[4-(2-chloro-4-nitrophenyl)piperazin-1-yl][3-(2-methoxyphenyl)-5-methyl-1,2-oxazol-4-yl]methanone 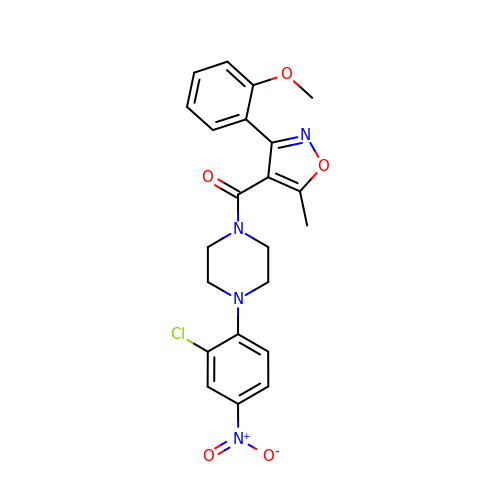| C22 H21 Cl N4 O5 | OQYUKAFYGKRXTK-UHFFFAOYSA-N>[4x]MRIPLVGKDSIESKDIGFTLIHEHLRVF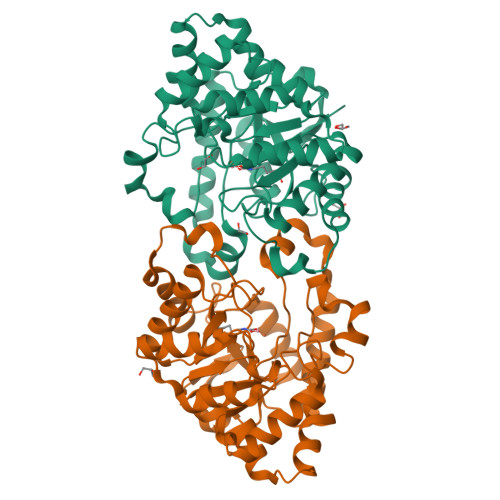SEAVRQQWPHLYNEDEEFRNAVNEVKRAMQFGVKTIVDPTVMGLGRDIRFMEKVVKATGINLVAGTGIYIYIDLPFYFLNRSIDEIADLFIHDIKEGIQGTLNKAGFVKIAADEPGITKDVEKVIRAAAIANKETKVPIITHSNAHNNTGLEQQRILTEEGVDPGKILIGHLGDTDNIDYIKKIADKGSFIGLDRYGLDLFLPVDKRNETTLRLIKDGYSDKIMISHDYCCTIDMGTAKPEYKPKLAPRWSITLIFEDTIPFLKRNGVNEEVIATIFKENPKKFFS>IDQKEKELIKESWKRIEPNKNEIGLLFYANLFKEEPTVSVLFQNPISSQSRKLMQVLGILVQGIDNLEGLIPTLQDLGRRHKQYGVVDSHYPLVGDCLLKSIQEYLGQGFTEEAKAAWTKVYG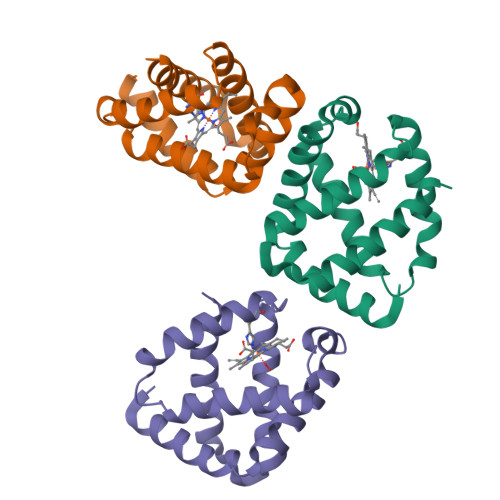IAAQVMTA[3x]> DNRDGNVYY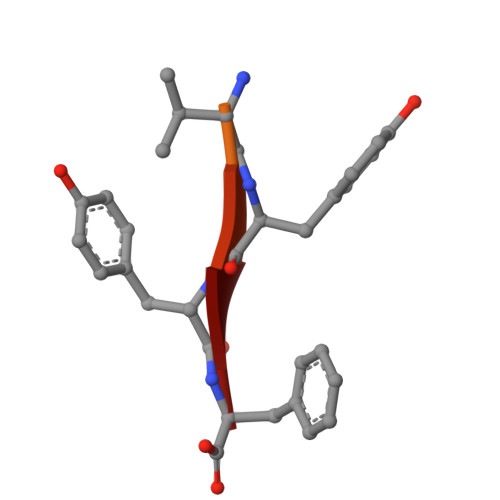F> MSSLKKILGLKGKGKKSKKLGIAPPPYEEDTSMEYAPSAPIDKSYFGVDEMDTYDPNQLRYEKFFFTVKMTVRSNRPFRTYSDVAAAVSHWDHMYIGMAGKRPFYKILAFLGSSNLKATPAVLADQGQPEYHAHCEGRAYLPHRMGKTPPMLNVPEHFRRPFNIGLYKGTIELTMTIYDDESLEAAPMIWDHFNSSKFSDFREKALMFGLIVEKKASGAWVLDSISH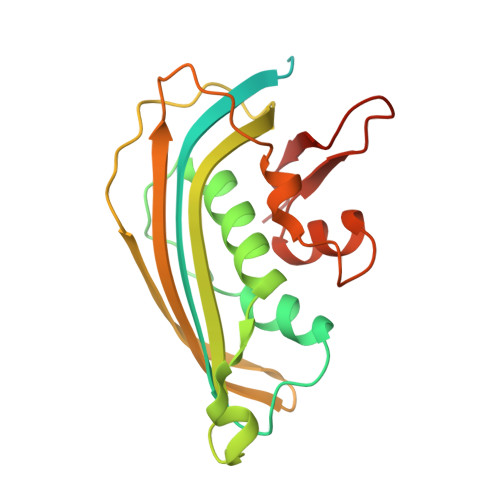FK>GPGSMAQSTIYSRVLGTGSYLPPNRVTNQDLAKRLAEQGIETSDEWIVARTGIHARYFAEPDVTTSDLAFIASQRAIEAADIDPQSIDLIIVATSTPDFVFPSTACLLQNKLGIRNHGAAFDVQAVCSGFAYAVATADSFIRSGQHRTALVIGAETFSRILDFKDRTTCVLFGDGAGAVILQASDEPGVLASALHADGSHSNILCTP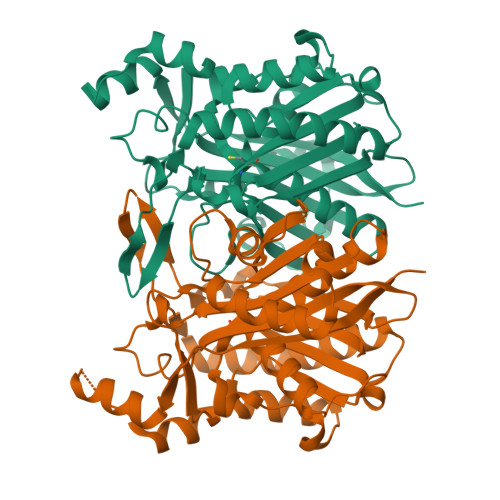GNVNGGVVSGSAFLHMDGQAVFKLAVNVLEKVAVEALEKANLSAEQIDWLIPHQANIRIMQSTCRKLGLPQERMIVTVGEHGNTSAASIPLALDVAVRDGRIKRGQNVLIEGVGGGFTWGASVIRY[4x]2-amino-6-methyl-7,8-dihydropteridin-4(3H)-one 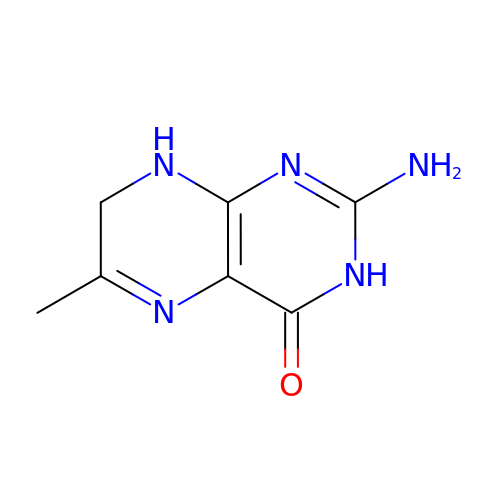| C7 H9 N5 O | ZGSZMKMOKGLFHK-UHFFFAOYSA-N> MATTTMTMIQALRSAMDVMLERDDNVVVYGQDVGYFGGVFRCTEGLQTKYGKSRVFDAPISESGIVGTAVGMGAYGLRPVVEIQF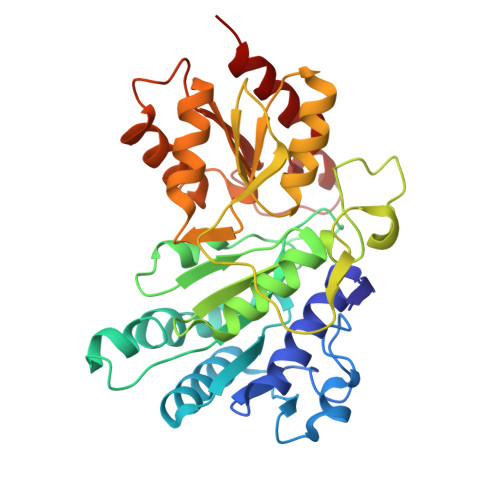ADYFYPASDQIVSEMARLRYRSAGEFIAPLTLRMPCGGGIYGGQTHSQSPEAMFTQVCGLRTVMPSNPYDAKGLLIASIECDDPVIFLEPKRLYNGPFDGHHDRPVTPWSKHPHSAVPDGYYTVPLDKAAITRPGNDVSVLTYGTTVYVAQVAAEESGVDAEVIDLRSLWPLDLDTIVESVKKTGRCVVVHEATRTCGFGAELVSLVQEHCFHHLEAPIERVTGWDTPYPHAQEWAYFPGPSRVGAALKKVMEV[3R-[3A,4A,5B(R*)]]-5-(1-CARBOXY-1-PHOSPHONOETHOXY)-4-HYDROXY-3-(PHOSPHONOOXY)-1-CYCLOHEXENE-1-CARBOXYLIC 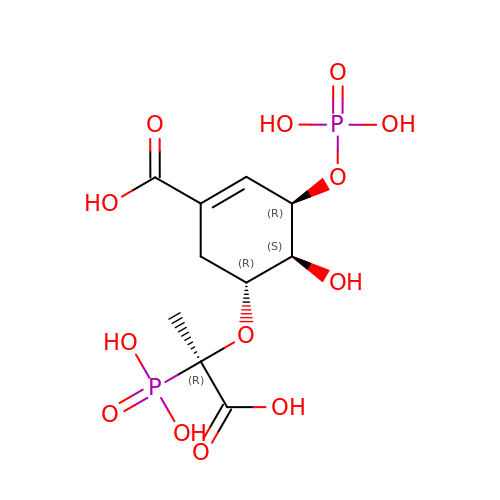ACID | C10 H16 O13 P2 | HUOJJMMXOWLGJU-QGOVLLJGSA-N> DGVGNASGDWHCDSTWMGDRVVTKSTRTWVLPSYNNHQYREIKSGSVDGSNANAYFGYSTPWGYFDFNRFHSHWSPRDWQRLINNYWGFRPRSLRVKIFNIQVKEVTVQDSTTTIANNLTSTVQVFTDDDYQLPYVVGNGTEGCLPAFPPQVFTLPQYGYATLNRDNTENPTERSSFFCLEYFPSKMLRTGNNFEFTYNFEEVPFHSSFAPSQNLFKLANPLVDQYLYRFVSTNNTGGVQFNKNLAGRYANTYKNWFPGPMGRTQGWNLGSGVNRASVSAFATTNRMELEGASYQVPPQPNGMTNNLQGSNTYALENTMIFNSQPANPGTTATYLEGNMLITSESETQPVNRVAYNVGGQMATNNQSSTTAPATGTYNLQEIVPGSVWMERDVYLQGPIWAKIPETGAHFHPSPAMGGFGLKHPPPMMLIKNTPVPGNITSFSDVPVSSFITQYSTGQVTVEMEWELKKENSKRWNPEIQYTNNYNDPQFVDFAPDSTGEYRTTRPIGTRYLTRPL;> VIKELVVSAGESVQITLPKNEVQLNAYVLQEPPKGETYTYDWQLITHPRDYSGEMEGKHSQILKLSKLTPGLYEFKVIVEGQNAHGEGYVNVTVKPE

Adeno-associated viruses (AAVs) belong to the Dependoparvovirus genus within the Parvoviridae family. Because of the broad differences in their tissue tropism and transduction efficiency and the absence of pathology, AAVs are the promising vehicles for therapeutic gene delivery. Adeno-associated virus receptor (AAVR), which is a glycosylated protein containing five polycystic kidney disease (PKD) repeat domains in its extracellular portion, was recently identified as a key proteinaceous receptor for multiple AAV serotypes to employ the post-attachment events of viral entry. To dissect the divergent rules of engagements between multiple AAV serotypes with AAVR, we select two AAV serotypes, AAV1 and AAV5, and solve the atomic structures of their complexes with AAVR by cryo-EM.

The density maps at atomic resolution, in particular the density at the virus–receptor interface, revealed that PKD2 binds to AAV1 and PKD1 binds to AAV5. In contrast, PKD1 contacts the outer rim of the spike on the AAV5 capsid outwards the icosahedral threefold axis, which is on the opposite side of AAVR PKD2 bound to AAV1/AAV2, and spans the canyon region towards the icosahedral fivefold axis and the twofold/fivefold wall of the capsid. The AAVR PKD1 polypeptide spanning residues from AAVRV305 to AAVRE401 was built into the density and refined. PKD1 adopts an Ig-like fold and consists of two stacked antiparallel β-sheets containing nine stands. Each PKD1 molecule mainly contacts one AAV5 capsomer (named capsomer A) but makes one additional contact with an adjacent AAV5 capsomer (named capsomer B). The PKD1 residues in strands F/G and the CD loop interact with the AAV5 capsomers to form a major fulcrum. However, the structures of AAV5 capsomers with and without PKD1 attached display strict structural homology with an r.m.s.d of 0.27 Å for all Cɑ atoms from 519 residues, indicating that no obvious structural shift occurs upon AAVR binding. As a control, the wild-type (wt) AAVR bound to AAV5 with a KD value of 0.287 μM.3-[[2-pyridin-2-yl-6-(1,2,4,5-tetrahydro-3-benzazepin-3-yl)pyrimidin-4-yl]amino]propanoic 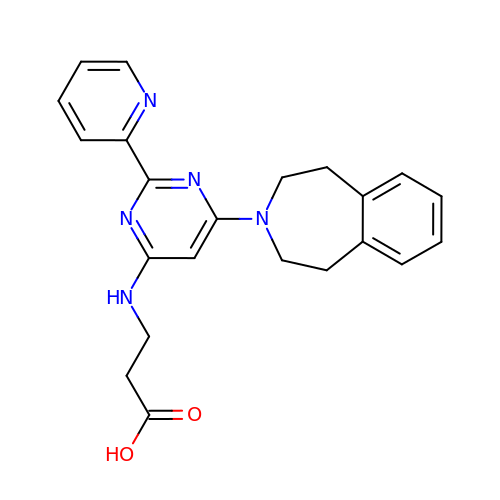acid | C22 H23 N5 O2 | AVZCPICCWKMZDT-UHFFFAOYSA-N> GSDPTQFEERHLKFLQQLGKGNFGSVEMCRYDPLQDNTGEVVAVKKLQHSTEEHLRDFEREIEILKSLQHDNIVKYKGVCYSAGRRNLKLIMEYLPYGSLRDYLQKHKERIDHIKLLQYTSQICKGMEYLGTKRYIHRDLATRNILVENENRVKIGDFGLTKVLPQDKEFFKVKEPGESPIFWYAPE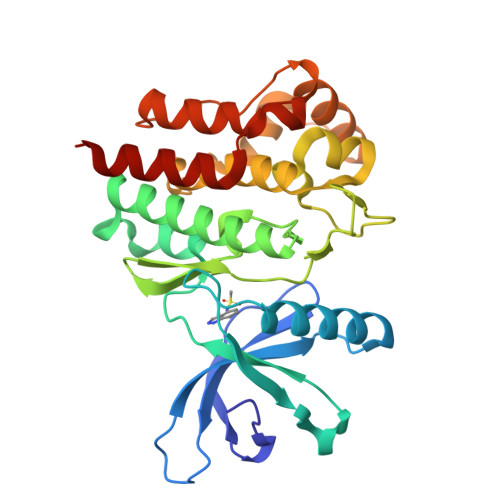SLTESKFSVASDVWSFGVVLYELFTYIEKSKSPPAEFMRMIGNDKQGQMIVFHLIELLKNNGRLPRPDGCPDEIYMIMTECWNNNVNQRPSFRDLALRVDQIRDNMAG>EPEPQMVLSPLTSAAIFLVVTIDSGGEDTVRDLLSDVASLERAVGFRAQPDGRLSCVTGIGSEAWDRLFSGARPAGLHPFRELDGPVHRAVATPGDLLFHIRASRLDLCFALATEIMGRLRGAVTPQDEVHGFKYFDERDMLGFVDGTENPTGAAARRAVLVGAEDPAFAGGSYAVVQKYLHDIDAWEGLSVEAQERVIGRRKMTDVELSDDVKPADSHVALTSVTGPDGSDLEILRDNMPFGSVGREEFGTYFIGYARTPEVTETMLERMFLGTASAPHDRILDFSTAVTGSLFFTPAADFLEDL[6x]

A widely applicable approach is the use of photocaged substrates, where the photocage is soaked into the crystal in advance and then activated using a laser pulse to provide uniform initiation of the reaction throughout the crystal. This work characterizes photocage release of nitric oxide and binding of this ligand to two heme protein systems, cytochrome c′-β and dye-decolourizing peroxidase B using a fixed target sample delivery system. In this work, we describe a thorough characterization of the application of the NO photocage N,N′-bis-(carb­oxy­methyl)-N,N′-di­nitroso-1,4-phenyl­enedi­amine (henceforth referred to as NO cage) to room-temperature microcrystals of two proteins: a gas binding cytochrome c′ (McCP-β) and a dye-decolourizing peroxidase B (DtpB). Laser parameters for photoactivation are systematically explored, and time-resolved structures over timescales ranging from 100 µs to 1.4 s using synchrotron and XFEL beamlines are described. We have demonstrated a sample and time efficient approach using fixed targets to carry out time-resolved SSX and SFX experiments with an NO photocage over the microsecond to second time regimes.

Comparison of these different structures revealed no significant changes in the binding geometry of NO or nearby residues in the heme pocket, meaning that only a two-state transition between unbound and bound states is observed. This suggests that any intermediate steps in the NO binding process must be complete on timescales of less than 100 µs. On binding to the heme, NO was observed to bind in an end-on fashion via the nitro­gen atom with an Fe—N distance of approximately 2.0–2.5 Å and an Fe—N—O angle of approximately 105–150°. The variability in these values occurs across the six independent heme groups within the crystallographic model and could represent either genuine differences in binding due to subtle differences in the crystalline environments or simply uncertainty in modelling a small ligand into the electron density features. A small shift in the side-chain position of Asn245 was observed compared with the ‘empty’ site structure in all six of the hemes, and at all laser powers and timepoints. For DtpB, the structure of the NO ferric heme complex of this or any other B-type DyP have not been previously determined, and thus we have demonstrated here that such a complex rapidly forms on exposure to NO after photocage release.>[2x]APQQINDIVHRTITPLIEQQKIPGMAVAVIYQGKPYYFTWGYADIAKKQPVTQQTLFELGSVSQTFTGVLGGDAIARGEIKLSDPTTKYWPELTAKQWNGITLLHLATYTAGGLPLQVPDEVKSSSDLLRFYQNWQPAWAPGTQRLYANSSIGLFGALAVKPSGLSFEQAMQTRVFQPLKLNHTWIN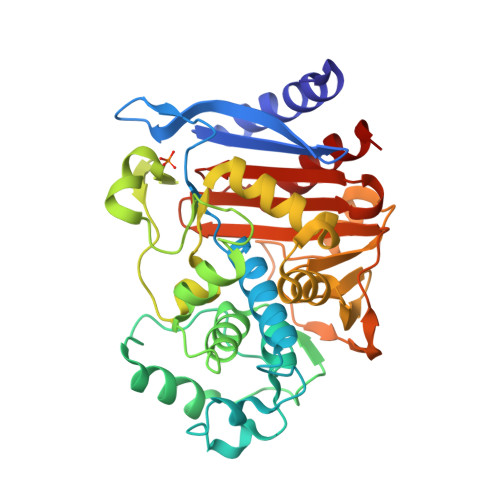VPPAEEKNYAWGYREGKAVHVSPGALDAEAYGVKSTIEDMARWVQSNLKPLDINEKTLQQGIQLAQSRYWQTGDMYQGLGWEMLDWPVNPDSIINGSDNKIALAARPVKAITPPTPAVRASWVHKTGATGGFGSYVAFIPEKELGIVMLANKNYPNPARVDAAWQILNALQ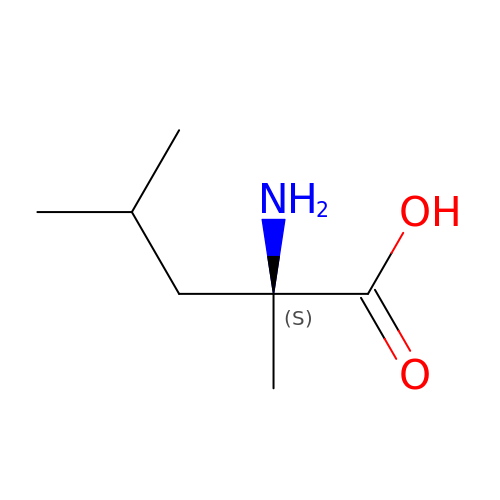2-METHYLLEUCINE | C7 H15 N O2 | ARSWQPLPYROOBG-ZETCQYMHSA-N Nucleoside diphosphate kinase A (NME1) is a multifunctional enzyme that was found to be pyrophosphorylated on Thr94 in human cells. A major role of NME1 is the synthesis of nucleoside triphosphates, other than ATP. NME1 catalyses this process by transferring the γ-phosphoryl group from ATP to a nucleoside diphosphate (NDP) via an active-site phosphohistidine intermediate. Oligophosphorylation was critically dependent on the catalytic histidine residue His118, and cryogenic electron microscopy analysis of the modified proteins suggests an intramolecular phosphoryl transfer mechanism.

For this, purified pS94-NME1 and ppS94-NME1 were vitrified, and cryo-EM datasets were recorded and refined to final resolutions of 2.8 Å for pS94-NME1 and 3.3 Å for ppS94-NME1. Notably, additional cryo-EM density at Ser94 was observed in both cases, which corresponds to the monophosphate or pyrophosphate group. The resulting model for pS94-NME1 revealed that the phosphoryl group is directed towards the His118 side chain, with a distance of 6.6 Å between the monophosphate group and the N1 of the His118 side chain (compared with 7.6 Å in wild-type NME1). Our hypothesis that NME1 oligophosphorylation proceeds via an intramolecular mechanism is supported by the cryo-EM data for phosphorylated, pyrophosphorylated and oligophosphorylated NME1. Both the phosphorylated and pyrophosphorylated side chains are oriented towards His118, with a distance that would be compatible with an intramolecular transfer. Even when the enzyme concentration was increased, the overall activity of pT94-NME1 was approximately 100-fold decreased compared with wild-type NME1, consistent with previous reports of a T94D mutant, which may be regarded as a phosphomimetic. The activity profile of pS94-NME1 was very similar to that of pT94-NME1, reduced approximately 100-fold compared with wild-type NME1, suggesting that the pS94 mutation is a suitable substitute for pT94. To validate this hypothesis, pS94-NME1 was freshly expressed and analysed by MS/MS, indeed revealing the autocatalytic formation of a pyrophosphate group at Ser94, and the formation of oligophosphate chains at this position. By contrast, neither wild-type NME1 nor the double mutant pS94-NME1(H118F) showed any higher phosphorylation states. These observations suggest an autocatalytic phosphoryl transfer between His118 and prephosphorylated Ser94, to generate the pyro- and oligophosphorylation states. In fact, when pS94-NME1 was treated with ATP, detection of the pyrophosphorylated intermediate was difficult because it appeared to subsequently convert to the tri- and tetraphosphorylated species at a much higher rate.

>[6x]MHHHHHHMANCERTFIAIKPDGVQRGLVGEIIKRFEQKGFRLVGLKFMQASEDLLKEHYVDLKDRPFFAGLVKYMHSGPVVAMVWEGLNVVKTGRVMLGESNPADSKPGTIRGDFCIQVGRNIIHGSDSVESAEKEIGLWFHPEELVDYTSCAQNWIYE>[4x]MATLSLTVNSGDPPLGALLAVEHVKDDVSISVEEGKENILHVSENVIFTDVNSI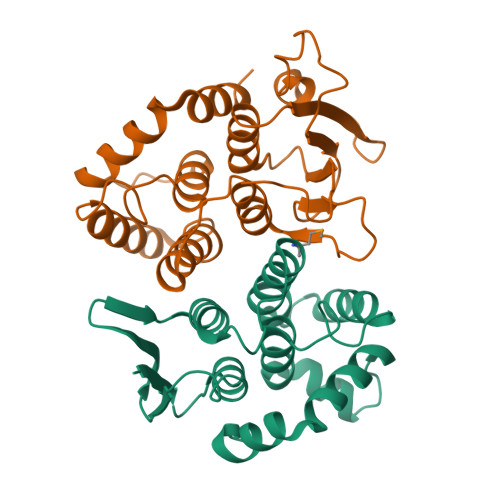LRYLARVATTAGLYGSNLMEHTEIDHWLEFSATKLSSSDSFTSTINELNHSLSLRTYLVGNSLSLADLSVWATLKGNAAWQEQLKQKKAPVHVKRWFGFLEAQQAFQSVGTKWDVSTTKAR;>[4x]MTNIIQADEPTTLTTNALDLNSVLGKDYGALKDIVINANPASPPLSLLVLHRLLCEHFRVLSTVHTHSSVKSVPENLLKCFGEQNKKQPRQDYQLGFTLIWKNVPKTQMKFSIQTMCPIEGEGNIARFLFSLFGQKHNAVNATLIDSWVDIAIFQLKEGSSKEKAAVFRSMNSALGKSPWLAGNELTVADVVLWSVLQQIGGCSVTVPANVQRWMRSCENLAPFNTALKLLKLEHHHHHH> GSHGTHAPLIHPLPHPIDLLALQQHDPARFPLLMESTASGTAQGRWSLLLVAQGDGLRLDADGQVRDQHDLVQPGTFLQALDRAWQHERLSHDGSHSLPFRGGWALMLDYEVASQIEPVLPARARGDGRPTALALRCPAAVLHDHHNEASFVIAEAGEQALLDALVALASAALPEAGQGWQPPQAVGEDAPQRFTDGVRRVIEYLRAGDVFQVNLSRRWNAQFAAPVSPQALYAQLRRANPAPFAGLFSAHGRHVVSSSPERLVSVHAGHAQTRPIAGTRPRFEGDDDAARIQELVGHPKERAEHVMLIDLERNDLGRICLPGTVVVDELMTVESYAHVHHIVSNVSGHLRPEVTPGEVIAATFPGGTITGCPKVRCMQIISELEQVPRGAYTGAFGWLNRDGDLDLNILIRTAEVDGHEVSFRTGAGIVVDSDPDKELDETRAKARGLLR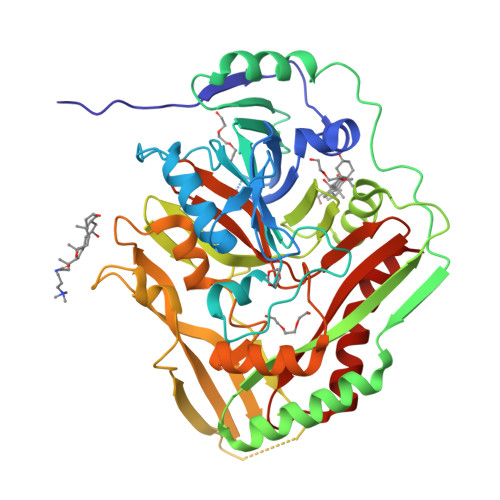ALGQQG>MQDNSRYTHFLTQHYDAKPQGRDDRYCE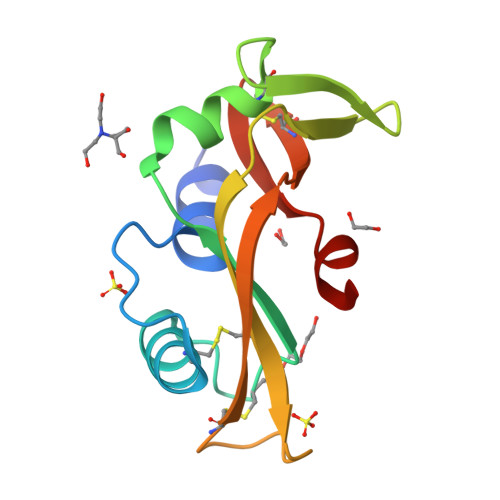SIMRRRGLTSPCKDINTFIHGNKRSIKAICENKNGNPHRENLRISKSSFPVTTCKLHGGSPWPPCQYRATAGFRNVVVACENGLPVHLDQSIFRRP[4x]>MEIRKKLVVPSKYGTKCPYTMKPKYITVHNTYNDAPAENEVNYMITNNNEVSFHVAVDDKQAIQGIPWERNAWACGDGNGPGNRESISVAICYSKSGGDRYYKAENNAVDVVRQLMSMYNIPIENVRTHQSWSGKYCPHR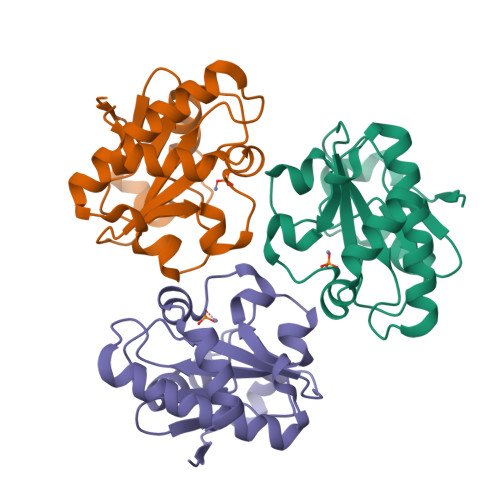MLAEGRWGAFIQKVKSGNVA[3x]~{N}-[(1~{R})-1-[3-azanyl-5-(trifluoromethyl)phenyl]ethyl]-7-methoxy-2-methyl-6-[(3~{S})-oxolan-3-yl]oxy-quinazolin-4-amine | 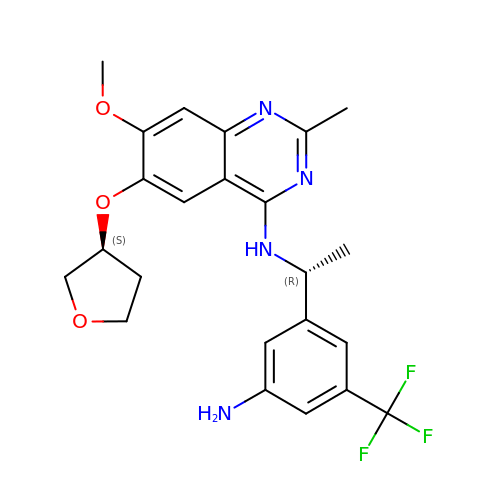C23 H25 F3 N4 O3 | XVFDNRYZXDHTHT-PXAZEXFGSA-N>[2x]GSHMSAPLPLDELRTFAEVLDRV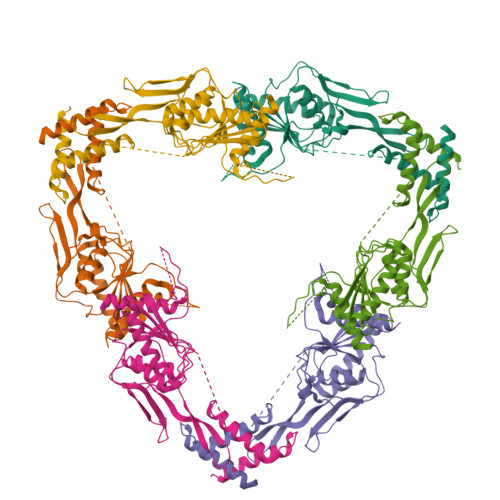KAAYVEPVDDKTLLENAIKGMLSNLDPHSAYLGPEDFAELQESTSGEFGGLGIEVGSEDGFIKVVSPIDDTPAARAGIQPGDLIVQIDGKPTKGQSMTEAVDSMRGKAGSPITLTIVRDGGRPFDVELKRAIIKVKSVKSQVLEPGYAYLRITQFQVNTGEEVVKALNQLRKDNKGRLKGLVLDLRNNPGGVLQSAVEVADAFLTKGLIVYTKGRIANSELRFSADPADPSDKVPLVVLINGGSAAAAEIVAGALQDQKRAILMGTDSFGKGSVQTVLPLNNDRALKLTTALYYTPNGRSIQAQGIVPDIEVGRAKVTQERSSFEGFKEADLQGHLANGNGGADRPTGKRAAPSERPQDSDYQLSQALSLLKGLSVTRG2-fluoro-6-{[2-(pyridin-2-yl)ethyl]amino}benzonitrile 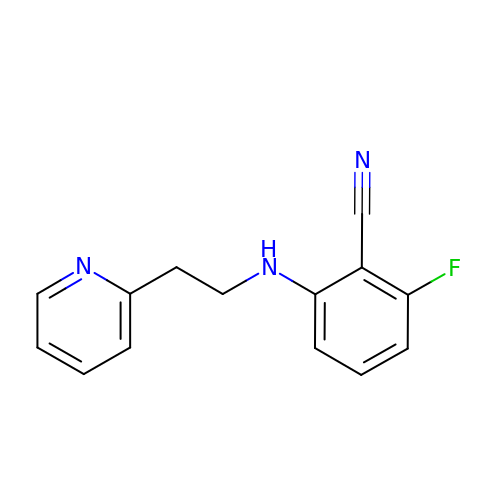| C14 H12 F N3 | YVRWCTBZWMJROU-UHFFFAOYSA-N> SGNAFPGDTRILVQINGTPQRVTLKELYELFNEEHYESMVYVRKKPKVDIKVYSFNPEEGKVVLTDIEEVIKAPATDHLIRFELELGSSFETTVDHPVLVYENGKFVEKRAFEVREGNIIIIIDESTLEPLKVAVKKIEFIEPPEDFVFSLNAKKYHTVIINENIVTHQ

Self-splicing protein introns (inteins) are genetic elements that are translated with their host proteins. After translation, the inteins catalyze their own excision and re-ligation of flanking protein regions (called exteins) with a peptide bond, resulting in active mature host proteins. There is a class of inteins lacking the HEN domain, so-called mini-inteins. We determined the crystal structure of a naturally occurring Pol-II mini-intein from Pyrococcus horikoshii and compared all three mini-inteins found in the genome of P. horikoshii.

We solved the three-dimensional structure of the PhoPol-II intein at a 1.48-Å resolution by molecular replacement. The crystal structure revealed the typical HINT fold with the β-strand insertion commonly observed among inteins from thermophilic organisms. In line with the loop minimization often observed for proteins from thermophiles, we could trace the electron densities for all of the 168 residues without detecting any flexible linker sequences, which were present in the structure of the PabPol-II intein. The relatively short helix of the PhoPol-II intein is rather reminiscent of a canonical mesophilic intein. Not surprisingly, the server returned the PabPol-II intein (2LCJ) as the closest structure, with a Z-score of 22.7, covering 164 residues with 1.5 Å-RMSD for Cα atoms. The largest difference between the two inteins lies in the flexible 19-residue sequence at the HEN insertion site for the PabPol-II intein, which is likely to be a remnant of HEN degradation during evolution. The sidechain of the C-terminal Gln166 in the PhoPol-II intein shows clear electron density, allowing the measurement of precise distances with other key residues. The distance between His154 and the carbonyl group of Q166 is 3.4 Å, which is shorter than the distance (4.6 Å) between the corresponding atoms of His160 in block F and the last residue, Asn172, in the PhoRadA intein structure. It appears that His154 stabilizes the side-chain conformation of Q166, making it less reactive towards the side-chain cyclization of Q166.> MGEKIKLEHGAGGEIMEELLRDVILKTLTLKSAGGIGLDALDDGATIPFGDKH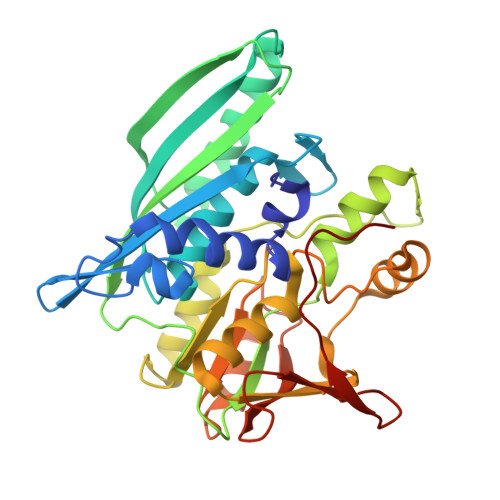IVFTIDGHTVKPLFFPGGDIGRLAVSGTVNDLAVMGAEPIALANSMIIGEGLDMEVLKRVLKSMDETAREVPVPIVTGDTKVVEDKIEMFVITAGIGIAEHPVSDAGAKVGDAVLVSGTIGDHGIALMSHREGIAFETELKSDVAPIWDVVKAVAETIGWENIHAMKDPTRAGLSNALNEIARKSNVGILVREADIPIRPEVRAASEMLGISPYDVANEGKVVMVVAREYAEEALEAMRKTEKGRNAAIIGEVIADYRGKVLLETGIGGKRFMEPPEGDPVPRIC> GMGTQLVMYEEEFTKINAVCDRLTKDANAKVVFLVDKNGQLISSAGQTQNIDTTSLASLTAGNVAAMGGLAK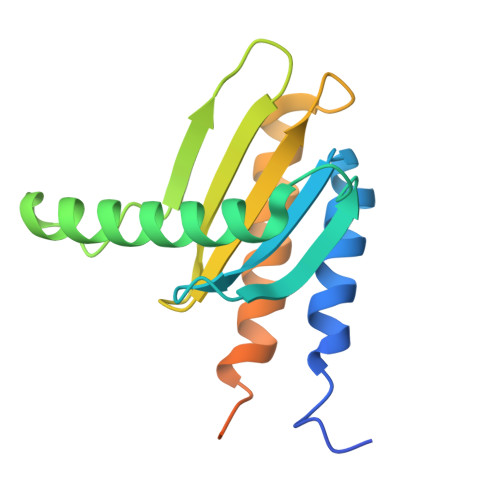LIGENEFPNQFHEGAKDSLYMTIVGSRVVLVVIFDNRTSLGLVRLRIKKASDELTKIFESLVKKTDSPGAGSPFAEISDDDIDNLFSE>MAPTFQTALFFTIISLSFAAPNAKQVRWCAISDLEQKKCNDLVGSCNVPDITLVCVLRSSTEDCMTAIKDGQADAMFLDSGEVYEASKDPYNLKPIIAEPYSSNRDLQKCLKERQQALAKKMIGHYIPQCDEKGNYQPQQCHGSTGHCWCVNAMGEKISGTNTPPGQTRATCERHELPKCLKERQVALGGDEKVLGRFVPQCDEKGNYEPQQFHGSTGYSWCVNAIGEEIAGTKTPPGKIPATCQKHDLVTTCHYAVAMVKKSSAFQFNQLKGKRSCHSGVSKTDGWKALVTVLVEKKLLSWDGPAKESIQRAMSKFFSVSCIPGATQTNLCKQCKGEEGKNCKNSHDEPYYGNYGAFRCLKEDMGDVAFLRSTALSDEHSEVYELLCPD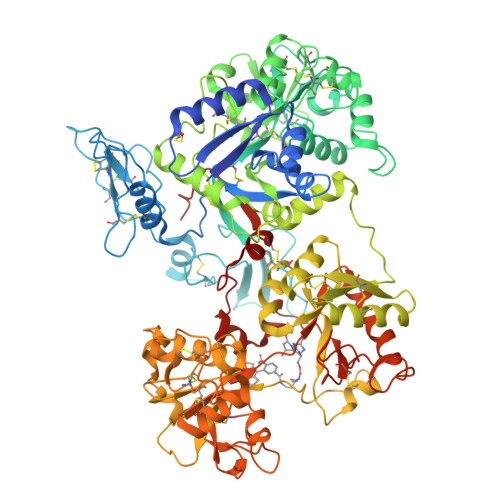NTRKPLNKYKECNLGTVPAGTVVTRKISDKTEDINNFLMEAQKRQCKLFSSAHGKDLMFDDSTLQLALLSSEVDAFLYLGVKLFHAMKALTGDAHLPSKNKVRWCTINKLEKMKCDDWSAVSGGAIACTEASCPKGCVKQILKGEADAVKLEVQYMYEALMCGLLPAVEEYHNKDDFGPCKTPGSPYTDFGTLRAVALVKKSNKDINWNNIKGKKSCHTGVGDIAGWVIPVSLIRRQNDNSDIDSFFGESCAPGSDTKSNLCKLCIGDPKNSAANTKCSLSDKEAYYGNQGAFRCLVEKGDVAFVPHTVVFENTDGKNPAVWAKNLKSEDFELLCLDGSRAPVSNYKSCKLSGIPPPAIVTREESISDVVRIVANQQSLYGRKGFEKDMFQLFSSNKGNNLLFNDNTQCLITFDRQPKDIMEDYFGKPYYTTVYGASRSAMSSELISACTIKHCSNSLEVLFQ[2x]Siderophore-binding proteins from two thermophilic bacteria, Geobacillus stearothermophilus and Parageobacillus thermoglucosidasius, were identified from a search of sequence databases, cloned and overexpressed. They are homologues of the well characterized protein CjCeuE from Campylobacter jejuni. The proteins have a two-domain structure, with the domains linked by a long α-helix at the base of the fold. The siderophore binding sites sit between the two domains.

In contrast to the Gst–azotochelin complex, the Pth–azotochelin complex was obtained by co-crystallization with iron(III)-azotochelin. All three Pth structures have considerably higher B values than those for Gst, with the azotochelin complex being the best ordered of the three. The three structures are closely similar to one another, with r.m.s.d.s of 0.43 and 0.48 Å compared with the apo form for the 5-LICAM and azotochelin complexes, respectively. The conserved iron-chelating residues in the three structures are His227 and Tyr288 in CjCeuE, His218 and Tyr279 in Gst and His215 and Tyr276 in Pth. The Fe atoms were coordinated by four O atoms from the two catecholate units of each ligand and the N and O donor atoms of conserved histidine and tyrosine residues, respectively, from the proteins. However, this is also true for the thermophilic proteins, where there is an even shorter ionic interaction between the azotochelin carboxyl and the equivalent arginine, but there is no difference in binding energy between azotochelin and 5-LICAM. In all three isomorphous structures there were difference density features associated with clear peaks in the anomalous difference maps which were modelled as nickel ions. The Ni1 and Ni4 sites in each structure lie on a crystallographic twofold axis and are linked through the sulfate ion. Ni3 and Ni5 are associated with the same protein side chains in the three structures but are remote from the siderophore binding site and do not interfere with ligand binding. These nickel cations and the associated sulfate anion are assumed to have been carried over from the nickel purification column.

> CGNEDNAKNASSSNPKNDSEEITIKHELGETKVKKKPEKVVVFDFGVLDSLDKLGVEVTGVPKANLPSYLEKYKDSKYENVGGLMEPDFEKINEIAPDLIIISGRQANSYEKFAEIAPTVYMGIDTKNYIDSFANNMKTLGKIFGKEKEVEKELESINKQIEAVKAKAEKTSGKALIVLTTGGKVSAYGPGSRFGIIHDVLGIKPVDANIEVSTHGQSISFEYIAEKNPDYLFVVDRDAVVAGKPSAKQTIENELVKKTNAYKNNRIIYLNPNYWYLAGGGLISVAEMINEVEKGIE>[2x]STAGKVIKCKAAVLWEEKKPFSIEEVEVAPPKAHEVRIKMVATGICRSDDHVVSGTLVTPLPVIAGHEAAGIVESIGEGVTTVRPGDKVIPLFTPQCGKCRVCKHPEGNFCLKNDLSMPRGTMQDGTSRFTCRGKPIHHFLGTSTFSQYTVVDEISVAKIDAASPLEKVCLIGCGFSTGYGSAVKVAKVTQGSTCAVFGLGGVGLSVIMGCKAAGAARIVGVDINKDKFAKAKEVGATE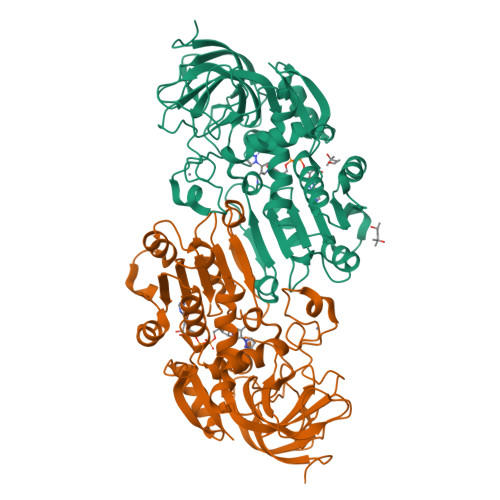CVNPQDYKKPIQEVLTEMSNGGVDFSFEVIGRLDTMVTALSCCQEAYGVSVIVGVPPDSQNLSMNPMLLLSGRTWKGAIFGGFKSKDSVPKLVADFMAKKFALDPLITHVLPFEKINEGFDLLRSGESIRTILTF>GAASATPDVDPDD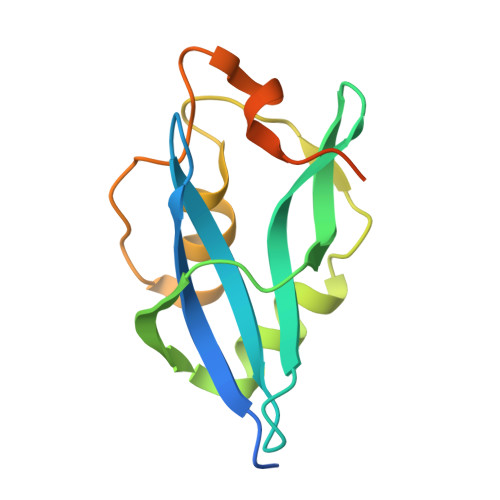RVYIVRAQRPTYVHWAIRKVAPDGSAKQISLSRSGIQALVALEPPEGEPYMEILPSHWTLAELQLGNKWEYSATNNCTHFVSSITGESLPNTGFSMALGIGALTAIAASAAVAVKALPGIRRQ[3x]>[2x]HHHHHHFNLPPGNYKKPKLLYCSNGGHFLRILPDGTV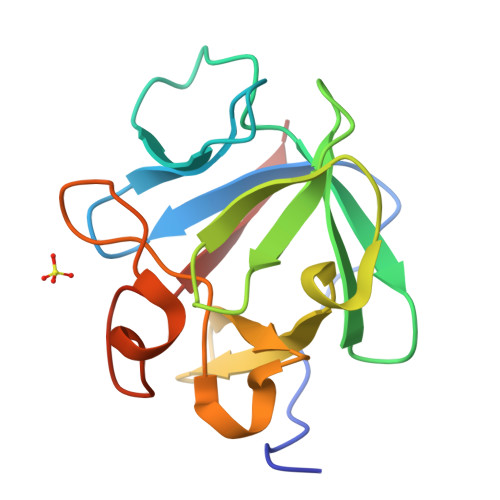DGTRDRSDQHIQFQLSAESVGEVYIKSTETGQYLAMDTDGLLYGSQTPNEECLFLERLEENHYNTYISKKHAEKNWFVGLKKNGSCKRGPRTHYGQKAILWLPLPVSSD> MAFSELLDQVGGLGRFQVLQTVALVVPIMWLCTQSMLENFSAAVPSHRCWVPLLDNSTAQASVPGALGPEALLAVSIPPGP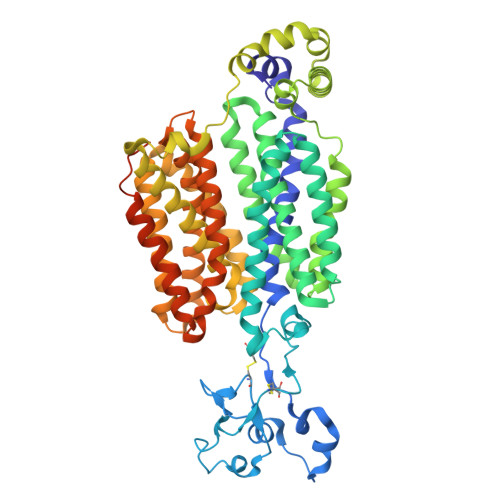NQGPHQCRRFRQPQWQLLDPNATATNWSEAATEPCVDGWVYDRSTFTSTIVAKWDLVCDSQALKPMAQSIYLAGILVGAAVCGPASDRFGRRLVLTWSYLQMAVSGTAAAFAPTFPVYCLFRFLVAFAVAGVMMNTGTLVMEWTSAQARPLVMTLNSLGFSFGHVLMAAVAYGVRDWALLQLVVSVPFFLCFVYSCWLAESARWLLITGRLDRGLRELQRVAAINGKRAVGDTLTPQVLLSAMQEELSVGQAPASLGTLLRTPGLRLRTCISTLCWFAFGFTFFGLALDLQALGSNIFLLQVLIGVVDIPAKIGTLLLLSRLGRRPTQAASLVLAGLCILANTLVPHEMGALRSALAVLGLGGLGAAFTCITIYSGELFPTVLRMTAVGLGQMAARGGAILGPLVRLLGVHGPWLPLLVYGTVPVLSGLAALLLPETQSLPAPDTIQDVQNQAVKKATHGTGNPSVLKSTQFSN>[2x]VGLTTLFWLGAIGMLVGTLAFAWAGRDAGSGERRYYVTLVGISGIAAVAYVVMALGVGWVPVAERTVFAPRYI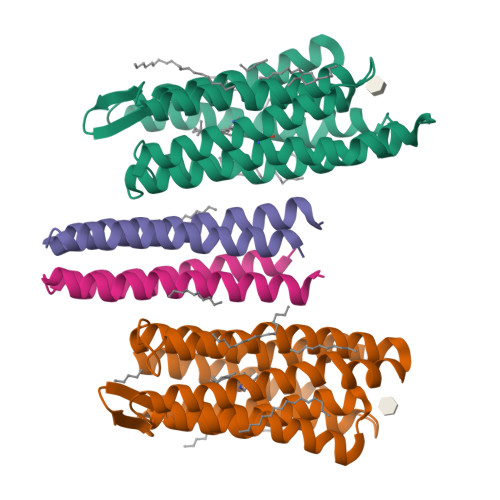DWILTTPLIVYFLGLLAGLDSREFGIVITLNTVVMLAGFAGAMVPGIERYALFGMGAVAFLGLVYYLVGPMTESASQRSSGIKSLYVRLRNLTVILWAIYPFIWLLGPPGVALLTPTVDVALIVYLDLVTKVGFGFIALDAAATLRAEHGESLAGVDTDAPAVADENSHHHHHHH;>AVSRLLLPSRVRHSYTGKMGAVFIFVGALTVLFGAIAYGEVTAAAATGDAAAVQEAAVSAILGLIILLGINLGLVAATLFGDTAASLSTLAAKASRMGDGDLDVELETRREDEIGDLYAAFDEMRQSVRTSLEDHHHHHHH[2x]In contrast, DEAD box protein 41 (DDX41), a member of the helicase superfamily 2 (SF2), is unique in that it can recognize two different types of ligands, double-stranded DNA (dsDNA) and CDN45. DDX41 consists of two RecA-like domains (i.e., DEAD and HELICc domains), which are conserved among DEAD box proteins. These domains have several conserved motifs, such as the Q motif and motif I, which are both essential for ATP binding by the DEAD box proteins. In this work, we determined two different crystal structures of the DDX41 DEAD domain in apo forms.

We determined the apo-form structures of two constructs, residues 169–402 (DEAD402) and 169–399 (DEAD399), at 1.5 and 2.2 Å resolutions, respectively. In the crystal structure of DEAD402, helix α2 and the Q motif are located adjacent to helix α3 and motif I, and the N-terminal residues (169–173) form a β strand (β1) and participate in the core β-sheet formation. We hereafter refer to this conformation of the N-terminal region as the “closed” form. The closed form of the DDX41 DEAD domain superimposes well on that of DDX3, with an RMSD of 1.56 Å over 215 Cα atoms. Especially, this superimposition revealed that the structure around the ATP-binding site, including the Q motif and motif I, adopts a similar conformation to that of DDX3. Interestingly, a malic acid molecule from the crystallization solution is present at this putative binding site for the ATP phosphate group in the closed form structure. One of the two carboxylate groups of the malic acid interacts with the main chain amide groups of motif I, while the other carboxylate group forms a salt bridge with the Arg residues in the adjacent molecule in the crystalline lattice. This observation is consistent with the fact that the crystals of the closed form were obtained only under conditions containing malic acid. Thus, in the present crystal structure, the DDX41 DEAD domain is trapped in the closed form by the carboxylate group of malic acid, which is bound by mimicking the phosphate group. Consequently, the structure of the ATP-binding site is completely rearranged in these open forms, and thus they do not seem to be able to bind ATP. Therefore, these results suggested that the closed form represents the ATP-bound state of DDX41, while both open forms 1 and 2 represent its nucleotide-free state.

> ILVEGDGIPPPIKSFKEMKFPAAILRGLKKKGIHHPTPIQIQGIPTILSGRDMIGIAFTGSGKTLVFTLPVIMFCLEQEKRLPFSKREGPYGLIICPSRELARQTHGILEYYCRLLQEDSSPLLRCALCIGGMSVKEQMETIRHGVHMMVATPGRLMDLLQKKMVSLDICRYLALDEADRMIDMGFEGDIRTIFSYFKGQRQTLLFSATMPKKIQNFAKSALVKPVTINVGRAG>[2x]MKKGVLIAFEGIDGSGKSSQATLLKDWIELKRDVYLTEWNSSDWIHDIIKEAKKKDLLTPLTFSLIHATDFSDRYERYILPMLKSGFIVISDRYIYTAYARDSVRGVDIDWVKKLYSF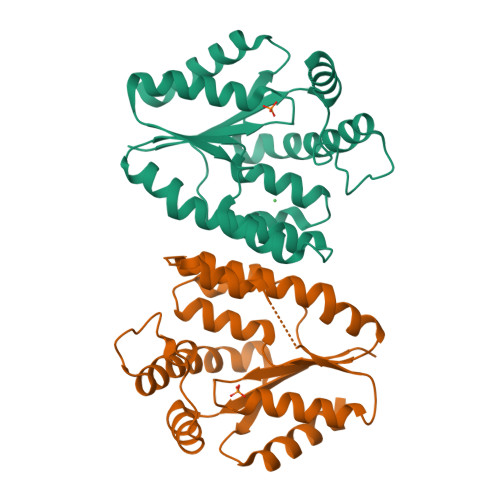AIKPDITFYIRVSPDIALERIKKSKRKIKPQEAGADIFPGLSPEEGFLKYQGLITEVYDKLVKDENFIVIDGTKTPKEIQIQIRKFVGELIDNSF> MHHHHHHDDDDKRTLPGEGTQVHPRAPLLQILKVAGAQEEVFTVKEVMHYLGQYIMMKQLYDKQRQHIVHCHDDPLGELLEV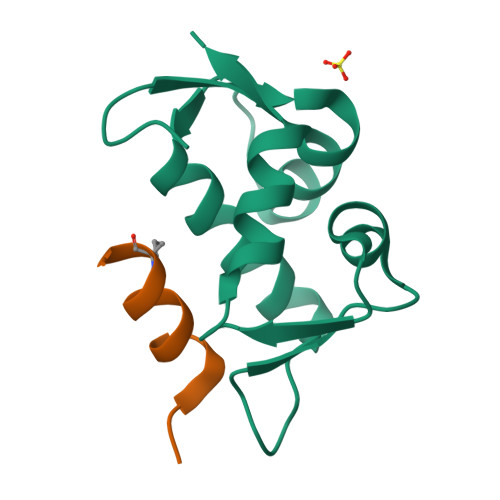GSFSVKNPSPLYEMLKRNLVIL;> LSQETFXDLWKLELENX>MTVTYTARVAKARFGGFSKLLLLWRGSIYKLLWRELLCFLGLFMALSAAYRFVLTEEQKRYFEKLVLYCDRYASLIPVSFVLGFYVTLVVHRWWNQYLSMPLTDALMCVVVGTVHGHDERGRLYRRTLMRYAGLSGVLILRSVSTAVFKRFPTIDHVVEAGFMTREERKKFENLN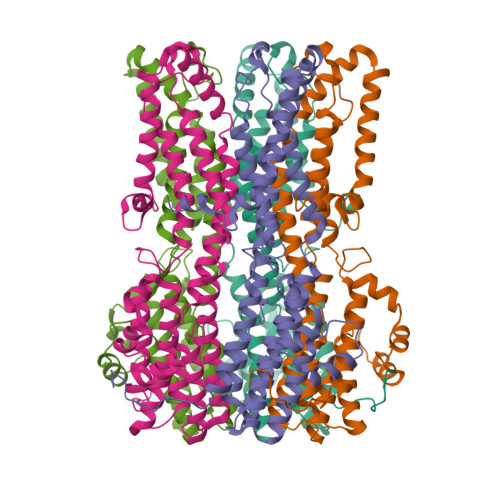SSYNKYWVPCVWFCNLAAQARREGRIRDNGAFKLLLEELNVFRSKCGMLFHYDWISVPLVYTQVVTIAVYSYFLACLIGRQFLDPAQGYKDHDLDLCVPIFTLLQFFFYAGWLKVAEQLINPFGEDDDDFETNFLIDRCFQVSMLAVDEMYDDLAMLEKDLYWDAAEARAPYTAATAFLMQQPSFQGSTFDITLAKEDMQFQRQDGLEAPLNEAHGDFLQRLLPVGTGMGTGGLL[5x]>EARLEEAVNRWVLKFYFHEALRAFRGSRYGDFRQIRDIMQALLVRPLGKEHTVSRLLRVMQCLSRIEEGENLDCSFDMEAELTPLESAINVLEMIKTEFTLTEAVVESSRKLVKEAAVIICIKNKEFEKASKILKKHMSKDPTTQKLRNDLLNIIREKNLAHPVIQNFSYETFQQKMLRFLESHLDDAEPYLLTMAKKAL[2x];>SRGLEVSHRLAPW[2x]

A Fanconi anemia (FA) protein, SLX4 (or BTBD12 or FANCP), is a molecular scaffold that interacts with structure-specific endonucleases XPF-ERCC1, MUS81-EME1, and SLX1. Shelterin consists of several proteins including duplex telomeric DNA-binding proteins TRF1 and TRF2 that anchor shelterin along the telomere repeats. The telomere restriction fragment homology (TRFH) domains of TRF1 and TRF2 directly recognize specific but distinct motifs on their interacting proteins. Here, we report the crystal structure of the TRF2-binding motif of SLX4 (SLX4TBM) in complex with the TRFH domain of TRF2 (TRF2TRFH) and map the interactions of SLX4 with endonucleases SLX1, XPF, and MUS81.

A short fragment of SLX4 consisting of residues 1014–1028 (SLX41014–1028) was sufficient for binding with TRF2TRFH with a KD of 750 nM, whereas binding enthalpy between SLX41014–1028 and TRF1TRFH was not measurable by ITC, indicating that SLX41014–1028 binding is specific for TRF2. SLX4TBM contains a modified sequence HxLxP that highly resembles the TRF2TRFH binding motif of Apollo (ApolloTBM), suggesting that SLX4TBM might bind to TRF2TRFH in the same fashion as ApolloTBM. We solved the crystal structure of the TRF2TRFH-SLX4TBM complex at 2.05 Å resolution. The structure exhibits a 2:2 stoichiometry between TRF2TRFH and SLX4TBM. Each SLX4TBM peptide adopts an extended conformation with a short one-turn helix at the N terminus and fits into the narrow groove formed by TRF2TRFH. Except for the very N terminus, SLX4TBM and ApolloTBM are identical in overall conformation. Two key hydrophobic residues in SLX4TBM, L1022, and P1024 bind to TRF2TRFH in the same fashion as do their counterparts in ApolloTBM. The imidazole ring of SLX4 H1020 occupies the same position as the side chain of Apollo Y504 in the ApolloTBM-TRF2TRFH complex. ITC data showed that alanine substitutions of these residues either completely abolished (SLX4 L1022A and TRF2 F120A) or substantially impaired (SLX4 H1020A and P1024A) the SLX4-TRF2 interaction. Hence, the observed SLX4-TRF2 interface is specific and necessary for both in vitro and in vivo binding of SLX4 to TRF2.> AQSVPWGISRVQAPAAHNRGLTGSGVKVAVLDTGISTHPDLNIRGGASFVPGEPSTQDGNGHGTHVAGTIAALNNSIGVLGVAPSAELYAVKVLGASGSGSVSSIAQGLEWAGNNGMHVANLSLGSPSPSATLEQAVNSATSRGVLVVAASGNSGA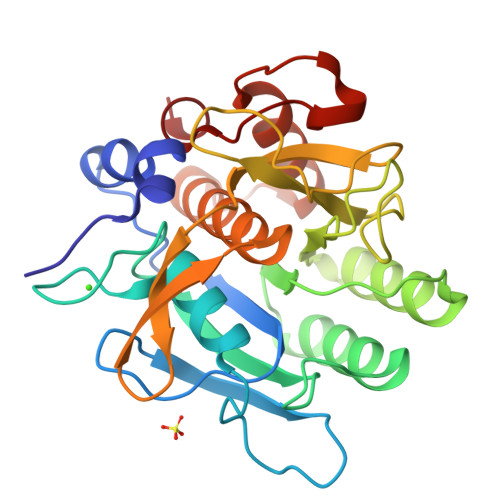GSISYPARYANAMAVGATDQNNNRASFSQYGAGLDIVAPGVNVQSTYPGSTYASLNGTSMATPHVAGVAALVKQKNPSWSNVQIRNHLKNTATGLGNTNLYGSGLVNAEAATR>[4x]MKITAARVIITCPGRNFVTLKI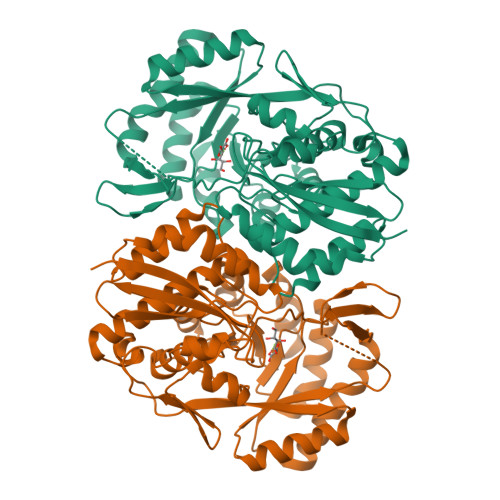ETDQGVYGIGDATLNGRELSVVAYLQEHVAPCLIGMDPRRIEDIWQYVYRGAYWRRGPVTMRAIAAVDMALWDIKAKMAGMPLYQLLGGRSRDGIMVYGHANGSDIAETVEAVGHYIDMGYKAIRAQTGVPGIKDAYGVGRGKLYYEPADASLPSVTGWDTRKALNYVPKLFEELRKTYGFDHHLLHDGHHRYTPQEAANLGKMLEPYQLFWLEDCTPAENQEAFRLVRQHTVTPLAVGEIFNTIWDAEDLIQNQLIDYIRATVVGAGGLTHLRRIADLASLYQVRTGCHGATDLSPVTMGCALHFDTWVPNFGIQEYMRHTEETDAVFPHDYWFEKGELFVGETPGHGVDIDEELAAKYPYKPAYLPVARLEDGTMWNW>KKIFKPE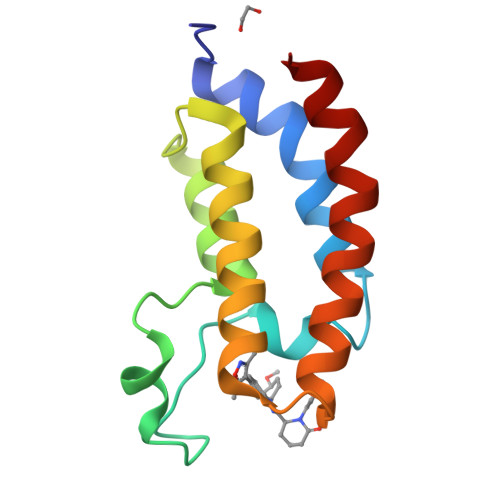ELRQALMPTLEALYRQDPESLPFRQPVDPQLLGIPDYFDIVKNPMDLSTIKRKLDTGQYQEPWQYVDDVWLMFNNAWLYNRKTSRVYKFCSKLAEVFEQEIDPVMQSLG[4x]> NQPYRTGFHFQPPKNWMNDPNGPMIYKGIYHLFYQWNPKGAVWGNIVWAHSTSTDLINWDPHPPAIFPSAPFDINGCWSGSATILPNGKPVILYTGIDPKNQQVQNIAEPKNLSDPYLREWKKSPLNPLMAPDAVNGINASSFRDPTTAWLGQDKKWRVIIGSKIHRRGLAITYTSKDFLKWEKSPEPLHYDDGSGMWQCPDFFPVTRFGSNGVETSSFGEPNEILKHVLKISLDDTKHDYYTIGTYDRVKDKFVPDNGFKMDGTAPRYDYGKYYASKTFFDSAKNR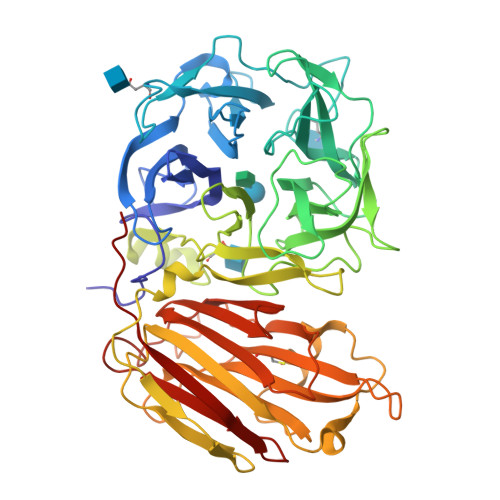RILWGWTNESSSVEDDVEKGWSGIQTIPRKIWLDRSGKQLIQWPVREVERLRTKQVKNLRNKVLKSGSRLEVYGVTAAQADVEVLFKVRDLEKADVIEPSWTDPQLICSKMNVSVKSGLGPFGLMVLASKNLEEYTSVYFRIFKARQNSNKYVVLMCSDQSRSSLKEDNDKTTYGAFVDINPHQPLSLRALIDHSVVESFGGKGRACITSRVYPKLAIGKSSHLFAFNYGYQSVDVLNLNAWSMNSAQIS HEXADECANE 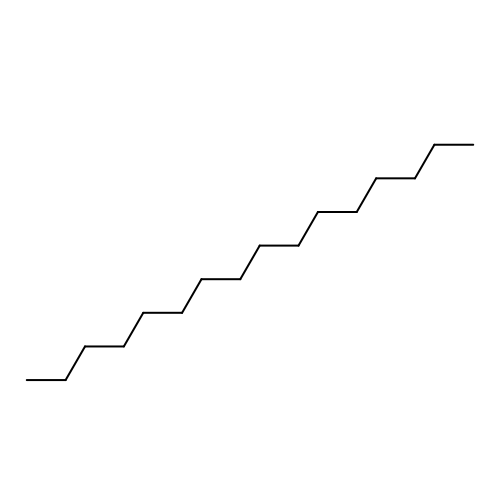| C16 H34 | DCAYPVUWAIABOU-UHFFFAOYSA-N>[2x]MAHHHHHHSLDAAAATLPRKSGSVDRLVRLAEADMAGVNRLITDRMQSDVAIIPALAEHLIAAGGKRLRPLMTVAAARLAGADNDHFQ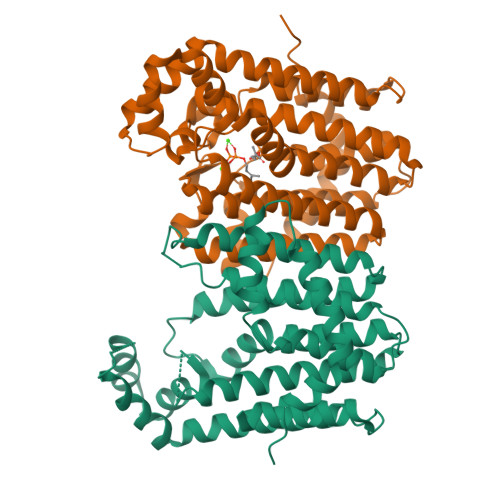KLAAAVEFIHTATLLHDDVVDGSQLRRGKVAAHLIWGGAQSVLVGDFLFARAFELMVETNSMKALEILARASRVIAEGEVLQLMRSHDLNLSQAVYLEIIQAKTAELFAAASEAGAVSAGVDVAKSEALRDYGLNLGLAFQLADDALDYGGATETLGKNAGDDFREGKATLPLLLAIARSGPREAEFWERAIGRREQTEADFRRARELIIGSGALDATLDLAADYADKAKAALAMFPANDWREALEELADFAVSRRA> FSIVGS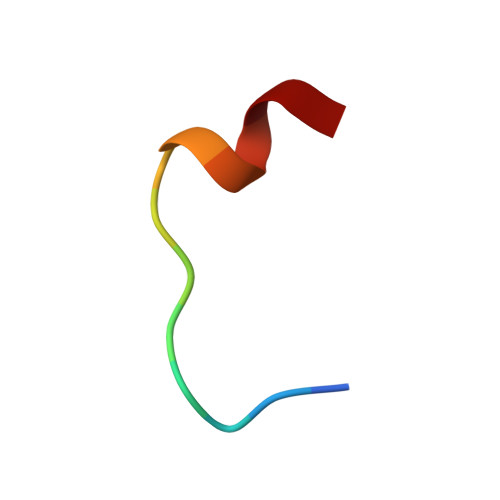LPRDFEL The lectin pathway of complement is activated by complexes comprising a recognition component (mannose-binding lectin, serum ficolins, collectin-LK or collectin-K1) and a serine protease (MASP-1 or MASP-2). MASP-1 activates MASP-2, and MASP-2 cleaves C4 and C4b-bound C2. MASPs are homodimers that circulate as zymogens bound to the collagenous domains of MBL. Each MASP comprises two N-terminal CUB (C1r/C1s, Uegf, and bone morphogenetic protein-1) domains separated by an epidermal growth factor (EGF)-like domain followed by two short complement regulator (SCR) domains and a C-terminal serine protease (SP) domain.

In particular, MASP-2 CUB1-EGF-CUB2 (subsequently called MASP-2 3D) was crystallized in the presence of citrate that chelates Ca2+, and although Ca2+ was bound to the EGF-like domain, the CUB1 and CUB2 domains lacked Ca2+ and became partially disordered as a result (Feinberg et al., 2003). Because there was no structure of rat MASP-1 3D, and the existing structure of rat MASP-2 3D lacked two of the three Ca2+, including those Ca2+ that form part of the binding site for MBL, both rat MASP-1 3D and MASP-2 3D were crystallized in the presence of 2 mM calcium and diffraction data were collected. This resulted in one MASP-1 structure at 3.7 Å resolution and three independent MASP-2 structures at 2.6–2.7 Å resolution. For MASP-2 3D, 279 of 280 residues were visible. Interestingly, the three structures overlaid closely, with RMSDs of 0.682, 0.871, and 0.992 Å over 276 Cα atoms. The only notable differences were in the N-terminal seven residues and in a loop within the EGF-like domain (Thr125–Ser130), probably reflecting flexibility. A major difference, however, was that the structures now contained three bound Ca2+ compared with the single Ca2+ in the EGF-like domain of the earlier MASP-2 3D structure. In the MASP-2 CUB1 domain, Ca2+ formed contacts with six oxygen atoms in the side chains of Glu48, Asp56, Asp101, and Asn104 and the main chain oxygen of Ser103 (distances between 2.3 and 2.7 Å). In the MASP-2 CUB2 domain, Ca2+ formed contacts with five oxygen atoms at the side chains of Glu215, Asp225, Asp262, and Ser264. The firm identification in this study of the three Ca2+ sites in rat MASP-2 now resolves a key ambiguity of the earlier rat MASP-2 structure (Feinberg et al., 2003).

> KWPEPVFGRLVSPGFPEKYGNHQDRSWTLTAPPGFRLRLYFTHFNLELSYRCEYDFVKLTSGTKVLATLCGQESTDTERAPGNDTFYSLGPSLKVTFHSDYSNEKPFTGFEAFYAAEDVDECRTSLGDSVPCDHYCHNYLGGYYCSCRVGYILHQNKHTCSALCSGQVFTGRSGFLSSPEYPQPYPKLSSCAYNIRLEEGFSITLDFVESFDVEMHPEAQCPYDSLKIQTDKREYGPFCGKTLPPRIETDSNKVTITFTTDESGNHTGWKIHYTSTAQ GLYCOLURIL | C4 H6 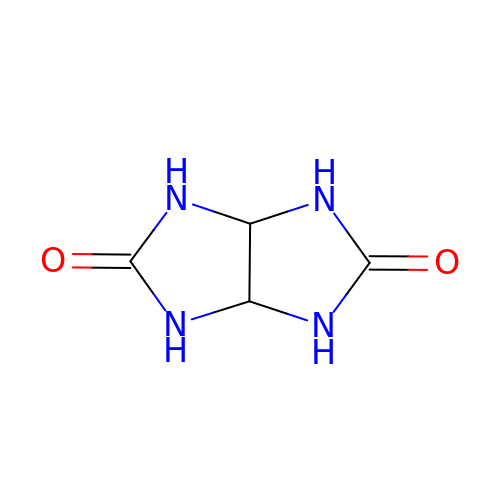N4 O2 | VPVSTMAPERLKKM-XIXRPRMCSA-N> PVRKQDTQRALHLLEEYRSKLSQTEDRQLRSSIERVINIFQSNLFQALIDIQEFYEVTLLDNPKLEVLFQGPGSDTGLYELLAALPAQLQPHVDSQEDLTFLWDMFGEKSLHSLVKIHEKLHYYEKQSP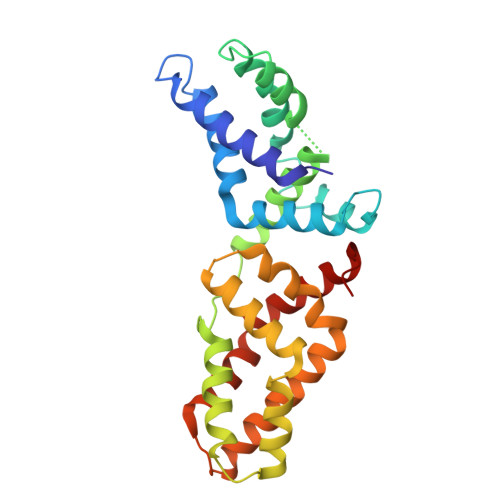VPILHGAAALADDLAEELQNKPLNSEIRELLKLLSKPNVKALLSVHDTVAQKNYDLEVLFQGPALGEPVRLERDICRAIELLEKLQRSGEVPPQKLQALQRVLQSEFCNAVREVYEHVYETVDIS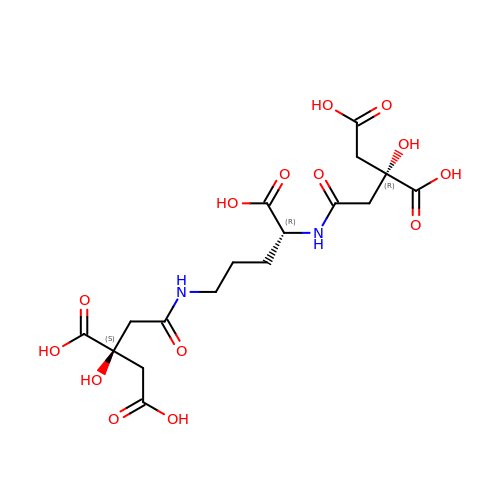(2R)-2-(2-{[(1R)-1-carboxy-4-{[(3S)-3,4-dicarboxy-3-hydroxybutanoyl]amino}butyl]amino}-2-oxoethyl)-2-hydroxybutanedioic acid | C17 H24 N2 O14 | VJSIXUQLTJCRCS-DFQXCPINSA-N> TTHYSVADRWGNAVSVTYTINASYGSAASIDGAGFLLNNEMDDFSIKPGNPNLYGLVGGDANAIEANKRPLSSMSPTIVLKNNKVFLVVGSPGGSRIITTVLQVISNV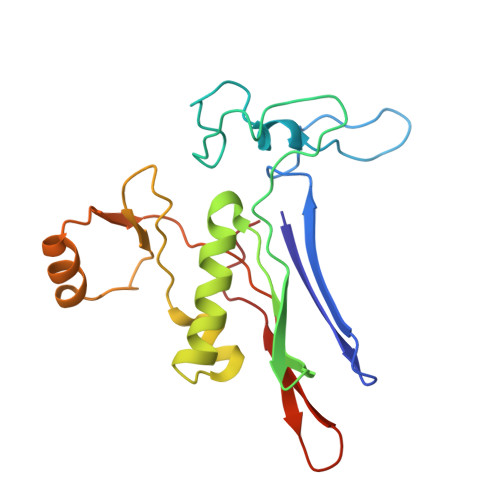IDYNMNISEAVSAPRFHMQWLPDELRIEKFGMPADVKDNLTKMGYQIVTKPVMGDVNAIQVLPKTKGSVFYGSTDPRKEF>[6x]HYTLPDLIANGTVAADWQFVRETANHYTNGPVTDVTDEAIRCYELDYSATPGETNIATVSAGSTVGMQGN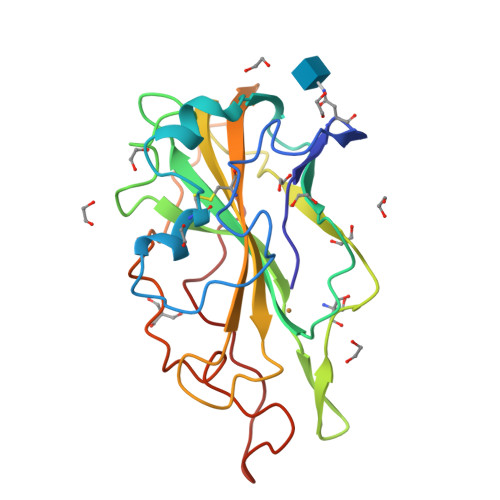GAFYHPGYFSAYLSQASPAANSPDAGTASTWFKIWEDPPVFENGALVFPSQSIDQVTFTIPKNLPSGQYLLRTEQIALHVASTFGGAQFYIGCAQLNVVDGGSGTPGPTVAFPGAYTGNEPGILINIYDLPAGYTGYQSPGPAVWQG> AHHHHHHMQGSVTEFLKPRLVDIEQVSSTHAKVTLEPLERGFGHTLGNALRRILLSSMPGCAVTEVEIDGVLHEYSTKEGVQEDILEILLNLKGLAVRVQGKDEVILTLNKSGIGPVTAADITHDGDVEIVKPQHVICHLTDENASISMRIKVQRGR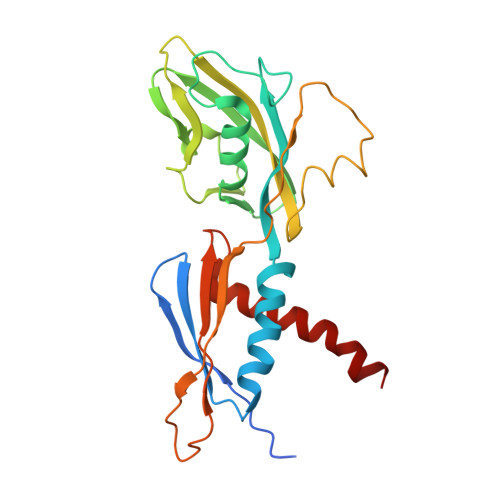GYVPASTRIHSEEDERPIGRLLVDACYSPVERIAYNVEAARVEQRTDLDKLVIEMETNGTIDPEEAIRRAATILAEQLEAFVDLR> IPVIEPLFTKVTEDIPGAEGPVFDKNGDFYIVAPEVEVNGKPAGEILRID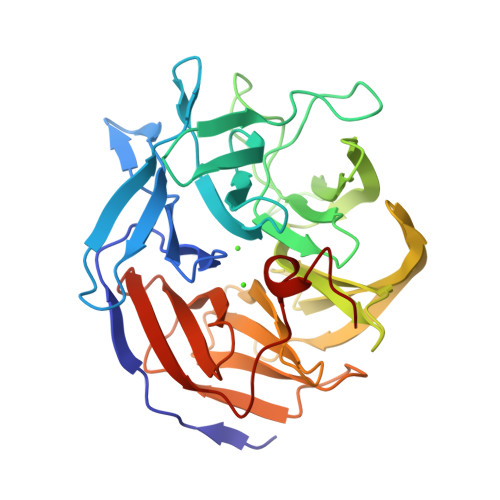LKTGKKTVICKPEVNGYGGIPAGCQCDRDANQLFVADMRLGLLVVQTDGTFEEIAKKDSEGRRMQGCNDCAFDYEGNLWITAPAGEVAPADYTRSMQEKFGSIYCFTTDGQMIQVDTAFQFPNGIAVRHMNDGRPYQLIVAETPTKKLWSYDIKGPAKIENKKVWGHIPGTHEGGADGMDFDEDNNLLVANYGSSHIEVFGPDGGQPKMRIRCPFEKPSNLHFKPQTKTIFVTEHENNAVWKFEWQRNGKKQYCETLKFGIF Multidrug resistance-associated protein 2 (MRP2) is an ATP-powered exporter important for maintaining liver homeostasis and a potential contributor to chemotherapeutic resistance. MRP2 is a single polypeptide comprising of an N-terminal transmembrane domain (TMD0) and the canonical transporter core of two transmembrane domains (TMD1 and TMD2) and two nucleotide-binding domains (NBD1 and NBD2). Using cryogenic electron microscopy (cryo-EM), we determine the structures of human MRP2 in three conformational states: an autoinhibited state, a substrate-bound pre-translocation state, and an ATP-bound post-translocation state.

We also analyzed the structure of a hydrolysis-deficient variant (E1462Q) in the presence of 5 mM ATP, which exhibited two conformations with approximately equal populations: an inward-facing, NBD-separated conformation and an NBD-dimerized conformation which we will discuss later. Because the structure of the E1462Q variant reveals more complete density of the R domain, we will discuss the inward-facing conformation based on this structure. The N-proximal half of the R domain (residues 861–893) forms a long loop along the inner surface of NBD1, extending nearly 90 Å into the TM cavity. Residues 894–897 form a sharp turn at the top of the TM cavity, and residues 898–918 form an α-helix between the two TM bundles. The remainder of the R domain extends into the cytosol and forms a short helical segment at the inner surface of NBD2. Near the apex of the TM cavity, the loop-turn-helix motif of the R domain engages in hydrogen bonding and extensive van der Waals interactions with TMD1 and TMD2. In addition, the C-proximal region of the R domain forms a composite ATP-binding site in conjunction with the Walker A/B motifs of NBD2. An ATP molecule is positioned between these two distant sequences and is stabilized by the canonical ATP-binding residues in NBD2, as well as by hydrogen bonds with R928 and K932 in the R domain. By sequestering the ATP-binding site in NBD2, the R domain of MRP2 competes directly with the signature sequence of NBD1, adding a new layer of control. At physiological ATP concentrations, ATP is likely bound at the interface of NBD2 and the R domain, further stabilizing the R domain in the auto-inhibitory position.

> MLEKFCNSTFWNSSFLDSPEADLPLCFEQTVLVWIPLGYLWLLAPWQLLHVYKSRTKRSSTTKLYLAKQVFVGFLLILAAIELALVLTEDSGQATVPAVRYTNPSLYLGTWLLVLLIQYSRQWCVQKNSWFLSLFWILSILCGTFQFQTLIRTLLQGDNSNLAYSCLFFISYGFQILILIFSAFSENNESSNNPSSIASFLSSITYSWYDSIILKGYKRPLTLEDVWEVDEEMKTKTLVSKFETHMKRELQKARRALQRRQEKSSQQNSGARLPGLNKNQSQSQDALVLEDVEKKKKKSGTKKDVPKSWLMKALFKTFYMVLLKSFLLKLVNDIFTFVSPQLLKLLISFASDRDTYLWIGYLCAILLFTAALIQSFCLQCYFQLCFKLGVKVRTAIMASVYKKALTLSNLARKEYTVGETVNLMSVDAQKLMDVTNFMHMLWSSVLQIVLSIFFLWRELGPSVLAGVGVMVLVIPINAILSTKSKTIQVKNMKNKDKRLKIMNEILSGIKILKYFAWEPSFRDQVQNLRKKELKNLLAFSQLQCVVIFVFQLTPVLVSVVTFSVYVLVDSNNILDAQKAFTSITLFNILRFPLSMLPMMISSMLQASVSTERLEKYLGGDDLDTSAIRHDCNFDKAMQFSEASFTWEHDSEATVRDVNLDIMAGQLVAVIGPVGSGKSSLISAMLGEMENVHGHITIKGTTAYVPQQSWIQNGTIKDNILFGTEFNEKRYQQVLEACALLPDLEMLPGGDLAEIGEKGINLSGGQKQRISLARATYQNLDIYLLDDPLSAVDAHVGKHIFNKVLGPNGLLKGKTRLLVTHSMHFLPQVDEIVVLGNGTIVEKGSYSALLAKKGEFAKNLKTFLRHTGPEEEATVHDGSEEEDDDYGLISSVEEIPEDAASITMRRENSFRRTLSRSSRSNGRHLKSLRNSLKTRNVNSLKEDEELVKGQKLIKKEFIETGKVKFSIYLEYLQAIGLFSIFFIILAFVMNSVAFIGSNLWLSAWTSDSKIFNSTDYPASQRDMRVGVYGALGLAQGIFVFIAHFWSAFGFVHASNILHKQLLNNILRAPMRFFDTTPTGRIVNRFAGDISTVDDTLPQSLRSWITCFLGIISTLVMICMATPVFTIIVIPLGIIYVSVQMFYVSTSRQLRRLDSVTRSPIYSHFSETVSGLPVIRAFEHQQRFLKHNEVRIDTNQKCVFSWITSNRWLAIRLELVGNLTVFFSALMMVIYRDTLSGDTVGFVLSNALNITQTLNWLVRMTSEIETNIVAVERITEYTKVENEAPWVTDKRPPPDWPSKGKIQFNNYQVRYRPELDLVLRGITCDIGSMEKIGVVGRTGAGKSSLTNCLFRILEAAGGQIIIDGVDIASIGLHDLREKLTIIPQDPILFSGSLRMNLDPFNNYSDEEIWKALELAHLKSFVASLQLGLSHEVTEAGGNLSIGQRQLLCLGRALLRKSKILVLDQATAAVDLETDNLIQTTIQNEFAHCTVITIAHRLHTIMDSDKVMVLDNGKIIECGSPEELLQIPGPFYFMAKEAGIENVNSTKF>[2x]GSHMMKRLVYISKISGHLSLEEIQRIGKVSIKNNQRDNITGVLLYLQGLFFQILEGENEKVDKLYKKILVDDRHTNILCLKTEYDITDRMFPNWAMKTINLNENSELMIQPIKSLLQTITQSHRVLEKYMPARVIYLINQGINPLTVEPQLVEKIIFFSDILAFSTLTEKLPVNEVVILVNRYFSICTRIISAYGGEVTKFIGDCVMASFTKEQGDAAIRTSLDIISELKQL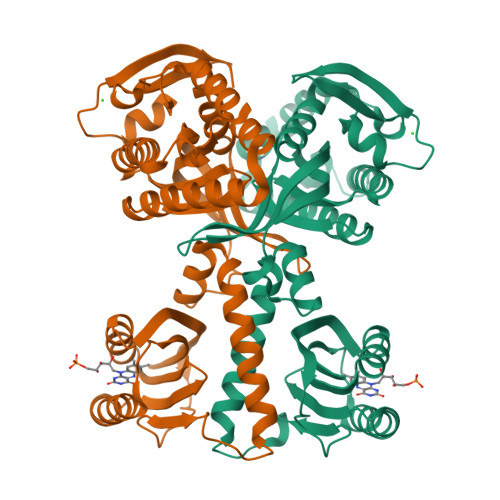RHHVEATNPLHLLYTGIGLSYGHVIEGNMGSSLKMDHTLLGDAVNVAARLEALTRQLPYALAFTAGVKKCCQAQWTFINLGAHQVKGKQEAIEVYTVNEAQKYYDTLQITQLIRQTLENDK>MAKVYKDLREFLEVLEQEGQLIRVKEEVNPEPDIAAAGRAAANLGKNQPAVFFEKIKGYKYSVVTNVHGSWQNHALMLGLDKNTSTKDQFYELNRRWDKFP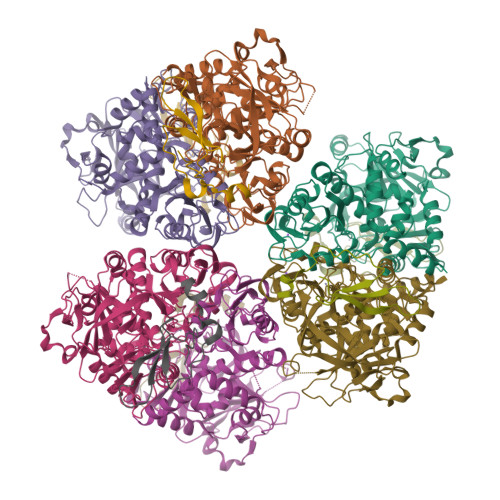VPPNVVKREAAPCKENVIDKDINLFEILPLYRINEQDGGFYISKASVVTADPEYPDDFNKLNVGTYRIQVKDRDRVGIQALAMHDIAVQLEKAEAENKPLPIAITIGNNPLVTFMASTPVGYNQNEYEFVGALQDGVPMDIVKSDLYDHLYVPAGSEVVLEGHIIPRVRTVEGPFGEFPGSYSGARLQCEVKIDRITHRTNPIFENLYLGIPWTEIDYLMALNTSVPLYKQLKETMPEVVAVNAMYTHGIGVIISTKVRYGGYAKGVAFRLLSTPHGMPYSKIVIVVDEFVDPFNLEQVMWALTTRVHPGKDVSIIENCPGMPLDPSTNPPGMHTKMIIDATTPVPPEPNPRETQLLDPPDGTEEWEEKLKELLKNQNR[6x];>[6x]MKCHRCGSDNVRKMVDSPVGDAWEVYVCEKCCYSWRSTENPVVMEKFKLDDNKIANMG>[2x]GALPDLKIEKLEEGVF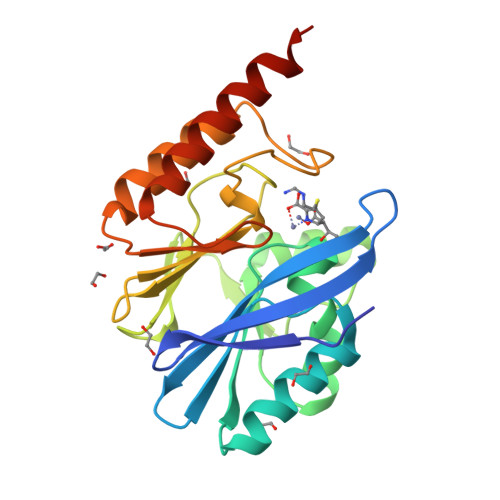VHTSFEEVNGWGVVTKHGLVVLVNTDAYLIDTPFTATDTEKLVNWFVERGYEIKGTISSHFHSDSTGGIEWLNSQSIPTYASELTNELLKKSGKVQAKYSFSEVSYWLVKNKIEVFYPGPGHTQDNLVVWLPESKILFGGCFIKPHGLGNLGDANLEAWPKSAKILMSKYGKAKLVVSSHSEKGDASLMKRTWEQALKGLKESKKTSSPSN> AAGAAPVDISTLPRVKVDLVKPPFVHAHDQVAKTGPRVVEFTMTIEEKKLVIDREGTEIHAMTFNGSVPGPLMVVHENDYVELRLINPDTNTLLHNIDFHAATGALG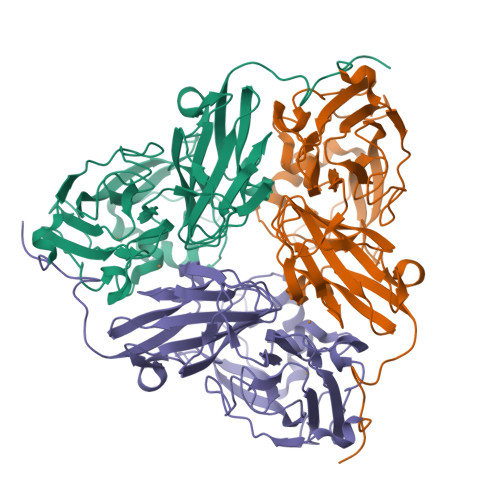GGALTQVNPGEETTLRFKATKPGVFVYHCAPEGMVPWHVTSGMNGAIMVLPRDGLKDEKGQPLTYDKIYYVGEQDFYVPKDEAGNYKKYETPGEAYEDAVKAMRTLTPTHIVFNGAVGALTGDHALTAAVGERVLVVHSQANRDTRPHLEGGHGDYVWATGKFRNPPDLDQETWLIPGGTAGAAFYTFRQPGVYAYVNHNLIEAFELGAAGHFKVTGEWNDDLMTSVVKPASM> CGRFAQSQTREDYLALLAEDIERDIPYDPEPIG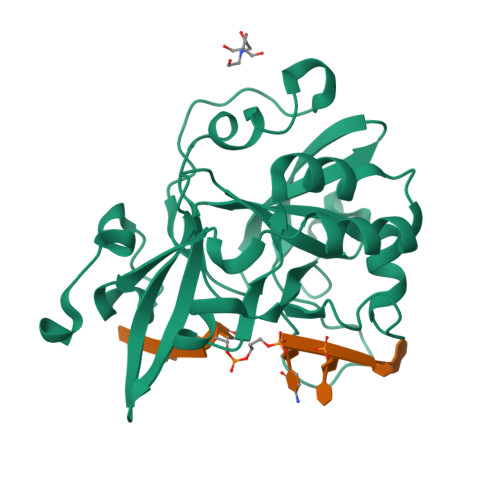RYNVAPGTKVLLLSERDEHLHLDPVFWGYAPGWWDKPPLINARVETAATSRMFKPLWQHGRAICFADGWFEWKKEGDKKQPFFIYRADGQPIFMAAIGSTPFERGDEAEGFLIVTAAADQGLVDIHDRRPLVLSPEAAREWMRQEISGKEASEIAASGCVPANQFSWHPVSRAVGNVKNQGAELIQPVLEVLF> MKTYALVMAGGRGERLWPLSR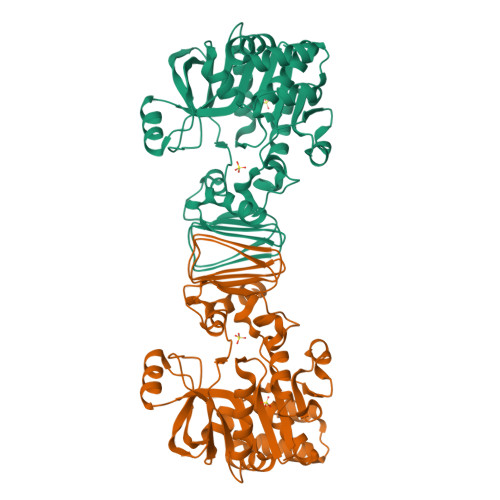EDRPKPFLPLFEGKTLLEATLERLAPLVPPERTLLAVRRDQEAVARPYADGIRLLLEPLGRDTAGAVLLGVAEALKEGAERLLVLPADHYVGDDEAYREALATMLEAAEEGFVVALGLRPTRPETEYGYIRLGPREGAWYRGEGFVEKPSYAEALEYIRKGYVWNGGVFAFAPATMAELFRRHLPSHHEALERLLAGASLEEVYAGLPKISIDYGVMEKAERVRVVLGRFPWDDVGNWRALERVFSQDPHENVVLGEGRHVALDTFGCVVYADRGVVATLGVSGLVVAKVGDEVLVVPKDWAREVREVVKRLEAQE>GPLGSVASAYAALPSWIAYEKARADLEEAKKNDVSPQLLKQLTKACNIAKSEFEREASVQKKLDKMAEQAAASMYKEARAVDRKSKIVSAMHSLLFGMLKKLDMSSVNTIIEQARNG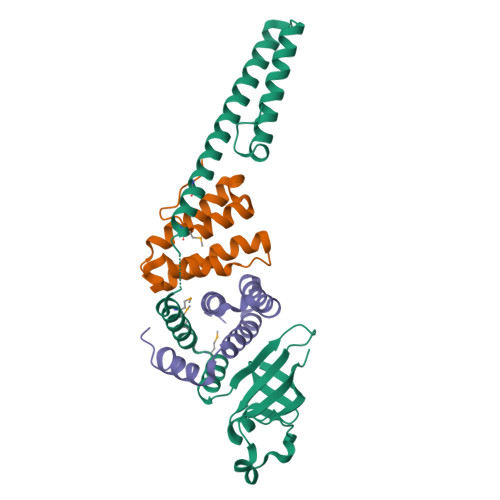VLPLSIIPAASATRLIVVTPNLEVLSKVRQENNVHYAGAIWSIVEVKDANGAQVHLKEVTAANELNITWPLSITCERTTKLQ[2x];>[4x]GPLGSKLTEMKCTNVVLLGLLSKMHVESNSKEWNYCVGLHNEINLCDDPDAVLEKLLALIAFFLSKHNTCDLSDLIESYFENTTILQ> MHHHHHHSAGLEVLFQGPVEQNWCVQPGLLEFGVGCSPLATLSVTNSFCSRQLIEVTCNVPDLVRISPSECYVSPDGGHAEIDVRLLRSPRQDLLEREPLIVVSMENERISVPISFKF

Spd-2/CEP192 proteins, defined by a conserved “Spd-2 domain” (SP2D) comprising two closely spaced AspM-Spd-2-Hydin (ASH) domains, play a critical role in centrosome assembly. The conserved centriole/centrosome protein Spd-2/CEP192 (fly/human nomenclature) plays an important part in mitotic centrosome assembly in humans, flies, and worms and also in the diverged centrosomes of Dictyostelium, which lack canonical centrioles. In flies and worms, the phosphorylation of Spd-2/SPD-2 at centrioles recruits Polo/Polo-like kinase 1 (PLK1), which then phosphorylates the large coiled-coil protein Cnn/SPD-5 to stimulate the assembly of a Cnn scaffold, and the internal molecular interactions that allow Cnn and SPD-5 to assemble into scaffolds are beginning to be elucidated. ASH domains are present in several proteins associated with centrosomes, cilia, flagella, and the Golgi complex, but the functions of these domains remain largely unknown.

An evolutionary analysis reveals that most Spd-2/CEP192 proteins contain additional ASH domains located close to the SP2D domain (one in Drosophila melanogaster and six in Homo sapiens; see Results). To partially validate the AF2 structural models, we solved the high-resolution structures of individual ASH domains from DmSpd-2 and H. sapiens CEP192 by crystallography (DmASH3 and HsASH7) to resolutions of 1.93 and 1.0 Å, respectively, or by nuclear magnetic resonance (NMR) spectroscopy (DmASH1). Instead, DmSP2D is essential for PCM scaffold assembly, a function that does not appear to require the additional ASH3 domain. Fusions in which the SP2D or its constituent individual ASH1 or ASH2 domains were deleted all failed to rescue the sterility of Spd-2−/− females, but the ASH3 deletion rescued this sterility nearly as well as the WT protein, although more variably. In contrast, Spd-2-∆ASH3-GFP was present at centrosomes at only slightly lower levels than WT Spd-2-GFP, and it appeared to be distributed more evenly between the centrioles and PCM than the WT protein. A 3D-SIM FRAP analysis suggested that Spd-2-∆ASH3-GFP was initially recruited to centrioles and then spread outward into the scaffold more quickly than the WT protein. The deletion of ASH3 did not significantly perturb the assembly of the residual scaffold in cnn−/− embryos, but the deletion of the SP2D, or of ASH1 or ASH2 individually, appeared to abolish the assembly of this residual scaffold. Collectively, these data indicate that the SP2D and ASH1 and ASH2 are required for Spd-2 and PCM scaffold assembly in vivo, while ASH3 is not. In flies, the single additional ASH domain is not essential for the Spd-2 function (as Spd-2-∆ASH3-GFP can rescue the female sterility of Spd-2 mutants) nor for Spd-2 scaffold assembly or for targeting Spd-2 to the centriole/centrosome.> MDVVSLDKPFMYFEEIDNELDYEPESANEVAKKLPYQGQLKLLLGELFFLSKLQRHGILDGATVVYIGSAPGTHIRYLRDHFYNLGVIIKWMLIDGRHHDPILNGLRDVTLVTRFVDEEYLRSIKKQLHPSKII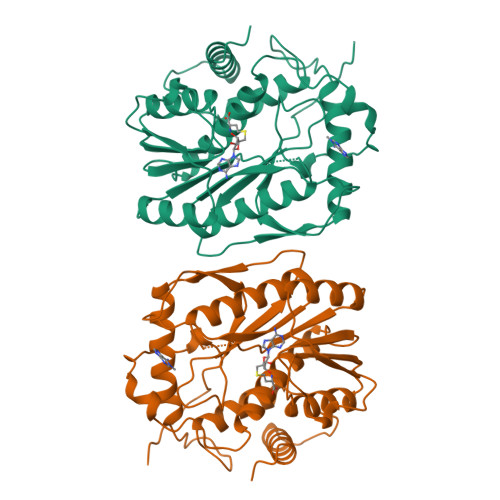LISDVRSKRGGNEPSTADLLSNYALQNVMISILNPVASSLKWRCPFPDQWIKDFYIPHGNKMLQPFAPSYSAEMRLLSIYTGENMRLTRVTKSDAVNYEKKMYYLNKIVRNKVVVNFDYPNQEYDYFHMYFMLRTVYCNKTFPTTKAKVLFLQQSIFRFLNIP>[2x]MVKPILYGI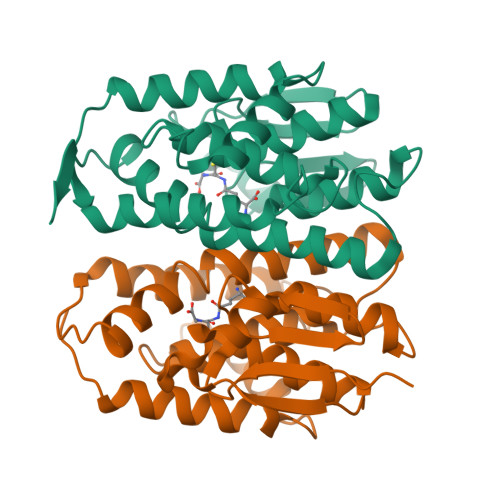DASPPVRAVKLTLAALQLPYDYKIVNLMNKEQHSEEYLKKNPQHTVPLLEDGDANIADSHAIMAYLVSKYGKDDSLYPKDLVKRALVDNRMYFESGVVFANALRSLAKMILFLGKTEVPQERIDAITEAYDFVEAFFKDQTYVAGNQLTIADFSLISSISSLVAFVPVDAAKYPKLSAWIKRLEQLPYYAENSTGAQQFVAAVKSKPFTVVGAENLYFQ> ETGEEPPRFIKEPKDQIGVSGGVASFVCQATGDPKPRVTWNKKGKKVNSQRFETIEFDESAGAVLRIQPLRTPRDENVYECVAQNSVGEITVHAKLTVLREDQLPSGFPNIDMGPQLKVVERT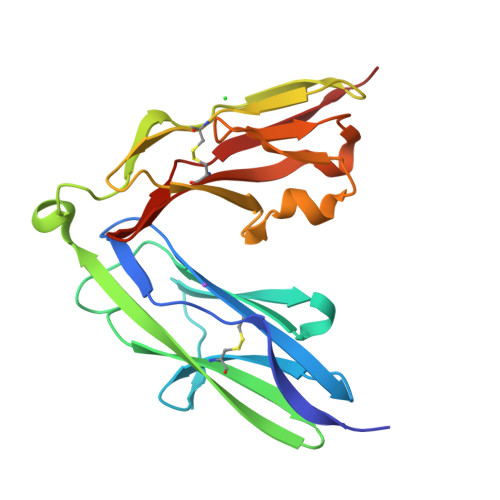RTATMLCAASGNPDPEITWFKDFLPVDPSASNGRIKQLRSGALQIESSEETDQGKYECVATNSAGVRYSSPANLYVRVR> GSVYPKELTQVFEHYINNNLFDIDSLVKFIEELGYNLEDLATLCLAHLLGYKKLEEPLKREDFLSTWFMQGCSTISDMQECIKTLDVKLHEDLQYFTQIYNYAFNLILDPNR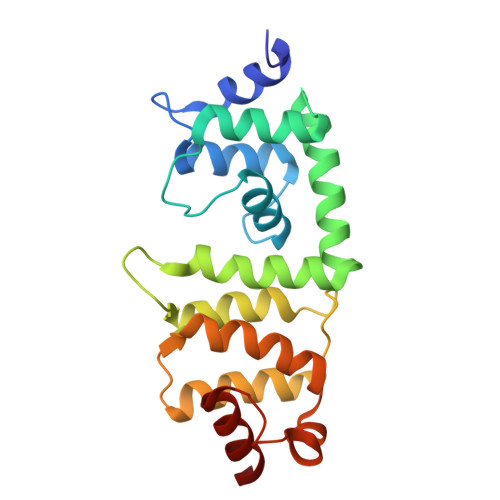KDIDTDEGIQYWKLFFQPEYPVRMEPDLLEAWFRFLRDEGKTTISKDTWRMLLLFFKRYPTIQKIISDYDETAAWPFIIDEFYECLQDQQ>SNADKSNKLQNLVAEQLVGCGFNEILNNSLTRAAYYDGLESYPSKNLVMLLNPLSADLNCMRQTLLFGGLESIAHNANRKNADLKFFEFGNCYHFDAEKKNPEKVLAPYSEDYHLGLWVTGKMVSNSWAHADENTSVYELKAYVENIFKRL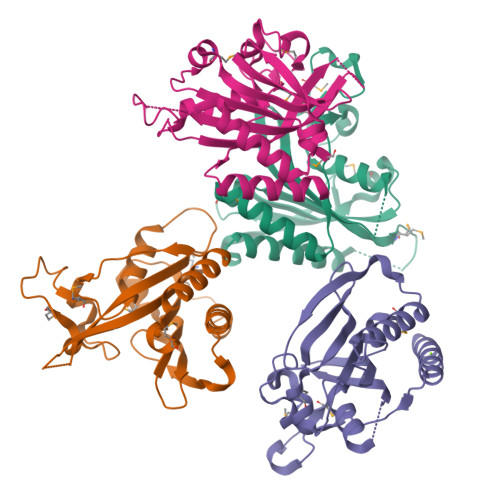GLDLHSLVVGNLSDDIYSTALTVNTKGGKRLATFGVVTKKMLKAFDVDNEVYYADLNWKELM[4x]> GHMDNLVLIRMKPDENGRFGFNVKGGYDQKMPVIVSRVAPGTPADLCVPRLNEGDQVVLINGR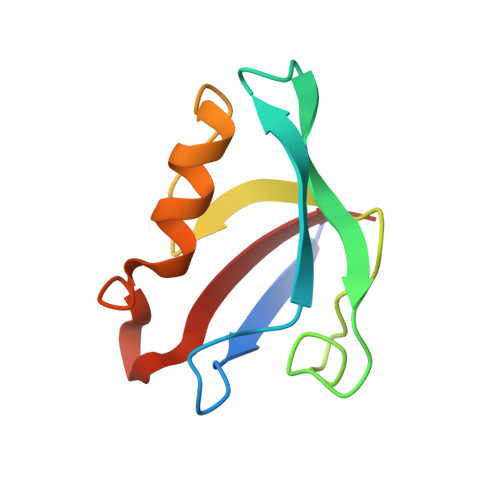DIAEHTHDQVVLFIKASCERHSGELMLLVRP The lipid-enveloped bacteriophages of the Cystoviridae family infect Gram-negative bacteria, mainly plant-pathogenic Pseudomonas species and share similarities with the members of the Reoviridae family, including bluetongue virus and rotavirus. Their genome of ∼14 kb consists of three dsRNA segments small (S), medium (M) and large (L), which are sequentially encapsidated as ssRNA precursors into the icosahedrally symmetric procapsid by the packaging NTPase P4 (15–23). P4 is a protein of ∼35 kDa, which can assemble into a hexameric ring. NTP-binding sites are located on the external perimeter of the ring at the interfaces between adjacent subunits, whereas the nucleic acid binding sites are found in the central channel. P4 proteins are the only known RNA-specific helicases belonging to helicase Superfamily 4 (SF4).

Of the P4s, only ɸ12 is purine specific, with pyrimidines also being accepted by ɸ16, ɸ18 and ɸ13. A specific feature in ɸ12 P4 is a hydrogen bond between the hydroxyl of S292 and N7 of the purine ring. The substitution S292A did not prevent ATP binding but completely abolished ATPase activity owing to misplacement of the triphosphate moiety in the active site. A displacement is also seen when the AMPcPP bound wild-type structure is compared with that of UTP bound hexamer. This confirms that pyrimidine triphosphates can bind the hexamer without being hydrolysed and should act as competitive inhibitors. Indeed, we find that UTP effectively competes with ATP and inhibits hydrolysis (data not shown). Hence, purine specificity is achieved by locking the base by hydrogen bonding to the N7 site of a purine. The correct coordination of the base results in the precise alignment of the nucleotide that is essential for catalysis so that UTP is misaligned and not hydrolysed.

>[3x]MIHLYDAKSFAKLRAAQYAAFHTDAPGSWFDHTSGVLESVEDGTPVLAIGVESGDAIVFDKNAQRIVAYKEKSVKAEDGSVSVVQVENGFMKQGHRGWLVDLTGELVGCSPVVAEFGGHRYASGMVIVTGKGNSGKTPLVHALGEALGGKDKYATVRFGEPLSGYNTDFNVFVDDIARAMLQHRVIVIDSLKNVIGAAGGNTTSGGISRGAFDLLSDIGAMAASRGCVVIASLNPTSNDDKIVELVKEASRSNSTSLVISTDVDGEWQVLTRTGEGLQRLTHTLQTSYGEHSVLTIHTSKQSGGKQASGKAIQTVIKNDELESVLRRLTSN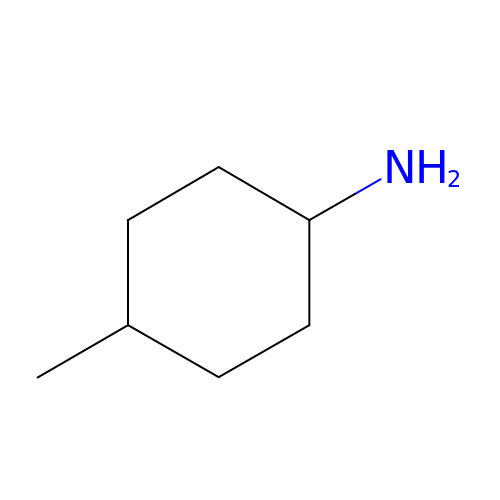trans-4-methylcyclohexanamine | C7 H15 N | KSMVBYPXNKCPAJ-LJGSYFOKSA-N> MRGSHHHHHHGMASMRILLSNDDGVHAPGIQTLAKALREFADVQVVAPDRNRSGASNSLTLESSLRTFTFDNGDIAVQMGTPTDCVYLGVNALMRPRPDIVVSGINAGPNLGDDVIYSGTVAAAMAGRHLGFPALAVSLNGYQHYDTA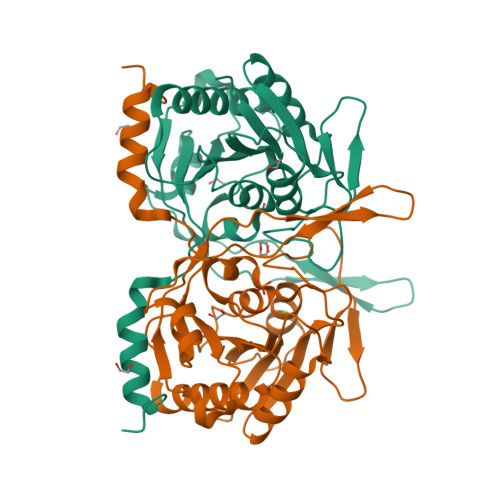AAVTCALLRGLSREPLRTGRILNVNVPDLPLAQVKGIRVTRCGSRHPADKVIPQEDPRGNTLYWIGPPGDKYDAGPDTDFAAVDEGYVSVTPLHVDLTAASAHDVVSDWLDSVGVGTQW> GGACAUGUAAUCGCGUGGAUAUG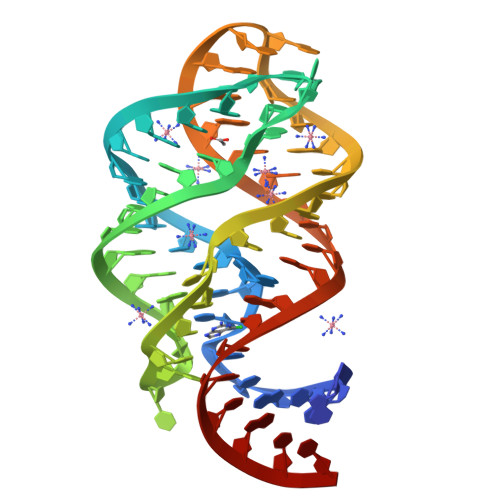GCACGCAAGUUUCUACCGGGCACCGUAAAUGUCCGACCAUGUCC> MRSCRRSVAQHPCAIQVDIVAMAAFISSFAGAQLAHARPSKQTALRAALTLPGTAETNLAVPSNAVRKVQPYPIAKPPSYSSVDSLRPARVSRMDADWATIYEQVRRQVMGNAYVMEGEAPDIDVAFSQLKGGNLTVREFVRAVGKSASYRTRFMEAKSSYNFVLLNFKHFLGRAPTQEEVSTHIQILATSGLEAEIDSYIDSDEYKALFGDHVVPYVVYRGTYLSSERFNRMVKANPGGATSDKAKSNLNMIATVAADLPTDAIDVMRGLPSPITSETLAFGTAYYWAKVEKEASEGRSASPIGEKIGKFDHAPISTYTSLCSYDKVNKAPQISVTNVGSDEHSYVSVTSKYIAPDMAAAAQMLADCQKYKAGGNAPTGKWMKYYPGTTVNMAPYISLNDTGSDSSRTVSVTLDKVKISPNKIGK;>[2x]MLDAFSRVVVNSDAKAAYVGGSDLQALKSFIADGNKRLDAVNSIVSNASCMVSDAVSGMICENPGLISPGGNCYTNRRMAACLRDGEIILRYVSYALLAGDASVLEDRCLNGLKETYIALGVPTNSSIRAVSIMKAQAVAFITNTATERKMSFAAGDCTSLASEVASYFDRVGAAIS

Red algae utilise a megadalton-size light harvesting antenna called the red algal phycobilisome (PBS)—comprised of rod structures formed from stacked, hexameric protein-pigment rings emanating from a protein core that is poised above an integral membrane photosystem. Published cryo-EM maps for two red algal phycobilisomes contain clusters of unmodelled density homologous to the cryptophyte-αβ protomer. We modelled these densities, identifying a new family of scaffolding proteins related to red algal phycobilisome linker proteins that possess multiple copies of a cryptophyte-α-like domain. These domains bind to, and stabilise, a conserved hydrophobic surface on phycoerythrin β, which is the same binding site for its primary partner in the red algal phycobilisome, phycoerythrin α.

One additional pair of ‘lone’ PE β subunits in the P. purpureum red algal PBS is attached to the C-terminal tail of the red algal PBS rod linker protein LR610 potentially providing stability. The C-terminal domain of LR6 that binds PE β in P. purpureum forms a flat structure comprised of a β ribbon followed by an α helix. Structural alignment of the C-terminal domain of LR6 to published cryptophyte-α subunits produced RMSD values ranging from 0.744 Å over 172 atoms to 1.335 Å over 208 atoms. This provided the first evidence for the existence of a cryptophyte-α-like protein in the red algal PBS. The only obvious difference between the two structures is the absence of a chromophore-binding loop in the C-terminal domain of LR6. Examination of the deposited cryo-EM maps confirms the structural similarity seen in the deposited model. Additionally, the map density shows that the N-terminal domain of the PE β subunit (not modelled in the original structure) has adopted a fold that has previously only been seen in cryptophyte-αβ protomers. One of these clusters is LR6, which includes a second CALM domain beyond the original model. For the unmodelled region of LR6 and most of the remaining two CaRSPs, we built de novo models including models for the metamorphic N-terminal domain of the associated PE β subunits. We hypothesise that the CALM domain originated in an early LR6 rod linker, by modification of the ancestral Pfam01383 domain, which allows it to bind to the metamorphic PE β (centre).>[30x]MGRGKVKPNRKSTGDNSNVVTMIRAGSYPKVNPTPTWVRAIPFEVSVQSGIAFKVPVGSL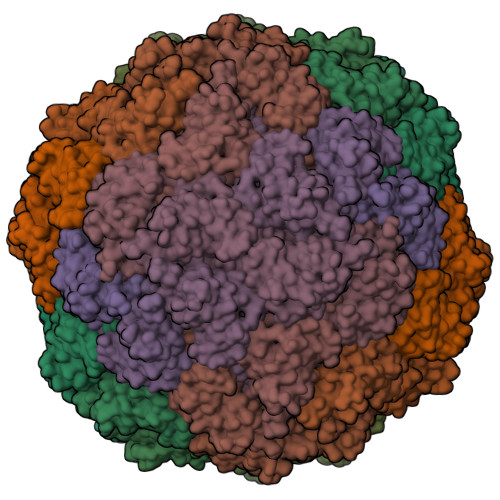FSANFRTDSFTSVTVMSVRAWTQLTPPVNEYSFVRLKPLFKTGDSTEEFEGRASNINTRASVGYRIPTNLRQNTVAADNVCEVRSNCRQVALVISCCFN(1S)-3-amino-1-[3-(cyclohexylmethoxy)phenyl]propan-1-ol | C16 H25 N O2 | 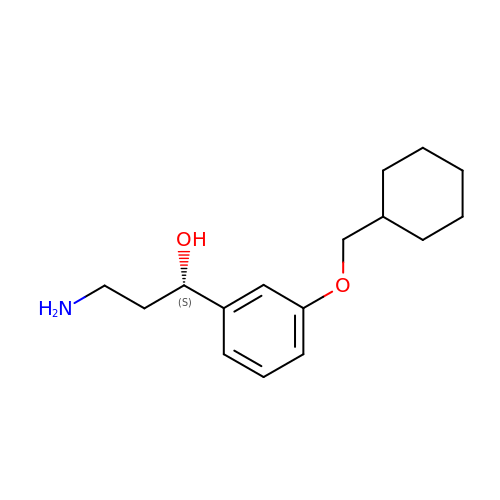WJIGGYYSZBWCGC-INIZCTEOSA-N>[2x]AAKTEQQIADIVNRTITPLMQEQAIPGMAVAVIYQGKPYYFTWGKADIANNHPVTQQTLFELGSVSKTFNGVLGGDAIARGEIKLSDPVTKYWPELTGKQWQGIRLLHLATYTAGGLPLQIPDDVRDKAALLHFYQNWQPQWTPGAKRLYANSSIGLFGALAVKPSGMSYEEAMTRRVLQPLKLAHTWITVPQNEQKDYAWGYREGKPVHVSPGQLDAEAYGVKSSVIDMARWVQ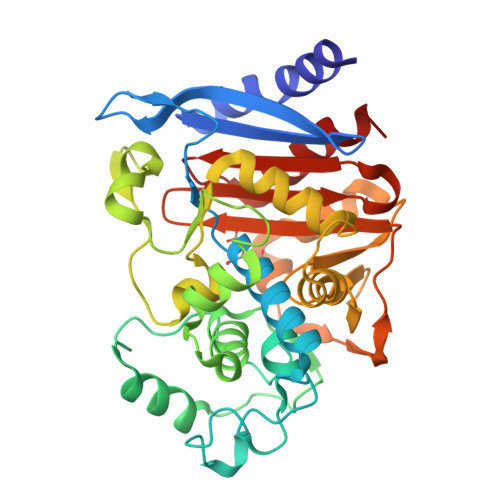ANMDASHVQEKTLQQGIALAQSRYWRIGDMYQGLGWEMLNWPLKADSIINGSDSKVALAALPAVEVNPPAPAVKASWVHKTGSTGGFGSYVAFVPEKNLGIVMLANKSYPNPVRVEAAWRILEKLQ> AIRLYKLAVALGVFIVSAPAFSHGHHSHGKPLTEVEQKAANGVFDDANVQNRTLSDWDGVWQSVYPLLQSGKLDPVFQKKADADKTKTFAEIKDYYHKGYATDIEMIGIEDGIVEFHRNNETTSCKYDYDGYKILTYKSGKKGVRYLFECKDPESKAPKYIQFSDHIIAPRKSSHFHIFMGNDSQQSLLNEMENWPTYY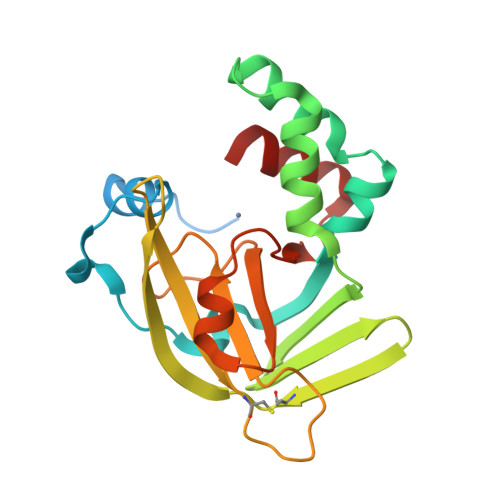PYQLSSEEVVEEMMSH To combat these defenses, Anopheles mosquitoes produce inhibitors belonging to the SG7 protein family that block complement at the alternative C3 convertase, C3bBb. Crystal structures of albicin and SG7.AF reveal a novel four-helix bundle arrangement that is stabilized by an N-terminal hydrogen bonding network. In this study, we describe the structures of albicin and its orthologs SG7.AF (from An. freeborni) and anophensin (from An. stephensi), characterize the binding and mechanism of AP inhibition by these inhibitors, and determine a role for properdin in modulating the inhibitory activity of SG7.AF. SG7 family members are quite similar to one another structurally, but amino acid sequence divergence suggests that specific side chain interactions are key determinants for the observed differences in target affinity.

Anophensin, the albicin ortholog from An. stephensi, has been shown to inhibit the contact pathway of coagulation through binding with factor XIIa and high-molecular-weight kininogen (29). We evaluated the AP inhibitory activity of recombinant anophensin in the erythrocyte lysis assay and found it to be much less potent than albicin or SG7.AF with an IC50 value of approximately 350 nM in NHS and 6 μM in PDS. We obtained crystals of a variant of anophensin containing three additional amino acids at its N-terminus. This variant exhibits a reduced retention volume in gel filtration chromatography suggesting oligomerization. The structure was then determined experimentally using a selenomethionine derivative and found to be significantly rearranged in that helix α1 is moved away from the rest of the helical bundle and forms part of a single extended alpha helical structure running from the N-terminus to the C-terminal end of α2. This presumably occurs due to loss of the stabilizing effect of the N-terminal hydrogen bonding network described above as a result of lengthening of the peptide and changing the position of the free N-terminal amino group. In the crystal, anophensin occurs as a symmetrical dimer in a domain-swapped arrangement where a number of the amino acid interactions in albicin between α1 and the rest of the bundle are retained but are now intermolecular. The extended coil region linking α1 and α2 also becomes helical, creating several new intermolecular interactions that may stabilize a dimeric form of the protein in solution. Dimerization in solution may account for the decreased gel filtration retention volume and reduced activity of this variant. Nevertheless, the anophensin structure with its extended N-terminus suggests that the α1-α2 region of the 30 kDa family might be unable to form the N-terminal hydrogen bonding network seen in albicin and SG7.AF and possibly assume a partially unfolded structure that could be relevant for the interaction with collagen.

>TEATRKHVQQLMKVFRAIDFDFTKKAFYLHRAKYGVQNQLRNPLYLKAMSLPRSAKLSQPCLNKMIDEVNDLESTFYAGFSFNCHDHDQYSMDCLEAAEPTYLDGLKKLAASTEQCLVQK[3x]> GPLGSQMTRQARHLYVGNIPFGITEEAMMDFFNAQMRLGGLTQAPGNPVLAVQINQDKN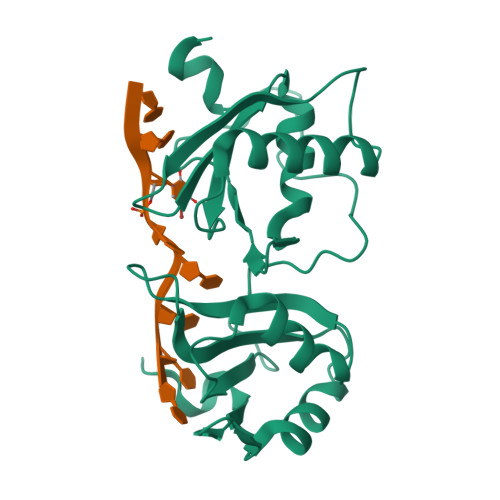FAFLEFRSVDETTQAMAFDGIIFQGQSLKIRRPHDYQPLPGMSENPSVYVPGVVSTVVPDSAHKLFIGGLPNYLNDDQVKELLTSFGPLKAFNLVKDSATGLSKGYAFCEYVDINVTDQAIAGLNGMQLGDKKLLVQRASVGAKN>[2x]M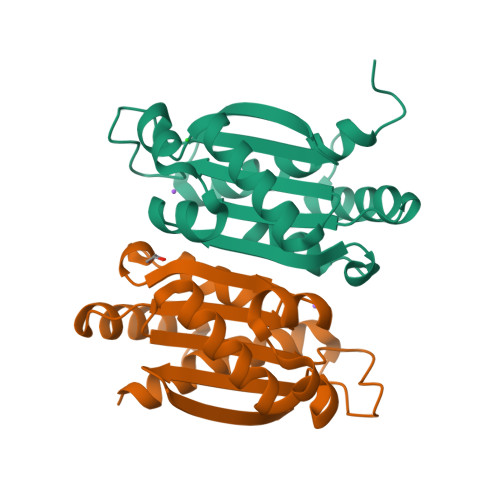SNLFHDSNNTVGELTKKLASKLTDLGLRLTTAESCTGGKLSVALCAEENTAEFYDVGLVVFSDEAKMRILGVRPETLERFTAVSEQTVTEMAASIRDIAQADISIAISGYAGPEGGDDGTAAGTVCFAWNIRGETETRTMLFSGDCQDVVEKAVHFSLAELLAALSDEDNG> MENKTETTVRRRRRIILFPVPFQGHINPILQLANVLYSKGFSITIFHTNFNKPKTSNYPHFTFRFILDNDPQDERISNLPTHGPLAGMRIPIINEHGADELRRELELLMLASEEDEEVSCLITDALWYFAQSVADSLNLRRLVLMTSSLFNFHAHVSLPQFDELGYLDPDDKTRLEEQASGFPMLKVKDIKSAYSNWQILKEILGKMIKQTKASSGVIWNSFKELEESELETVIREIPAPSFLIPLPKHLTASSSSLLDHDRTVFQWLDQQP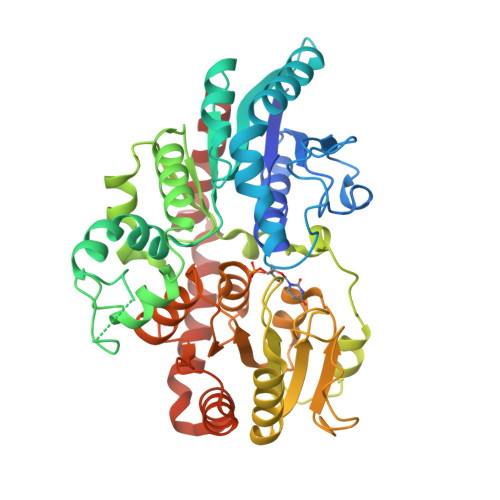PSSVLYVSFGSTSEVDEKDFLEIARGLVDSKQSFLWVVRPGFVKGSTWVEPLPDGFLGERGRIVKWVPQQEVLAHGAIGAFWTHSGWNSTLESVCEGVPMIFSDFGLDQPLNARYMSDVLKVGVYLENGWERGEIANAIRRVMVDEEGEYIRQNARVLKQKADVSLMKGGSSYESLESLVSYISSL> ADFLLDRMTPVSEEDIEGFAASTFKEVSDSKTATVI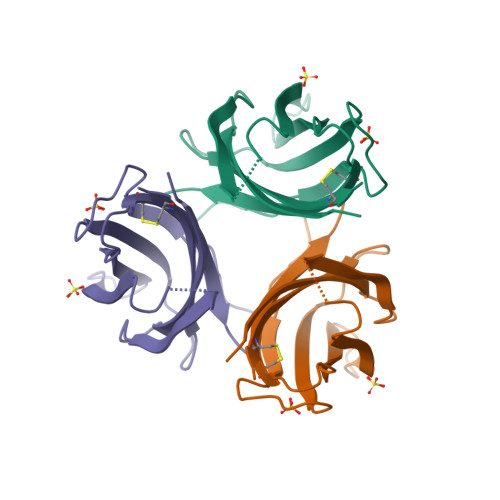VKADCETGDIDEVYNLAPSFGVTQEIKIYRSNNSSELDNVADSFHIYKISATDSDSGNTKKLLYGLRNKKAGYTCLCRIFAEIESDGIMANTNIGVAENNRDEIDENEEGKYGFLIPKQPAGAKLIIYFFLNCWT>[4x]SYTLPSLPYAYDALEPHFDKQTMEIHHTKHHQTFVNNANAALESLPEFANLPVEELITKLDQLPADKKTVLRNNAGGHANHSLFWKGLKKG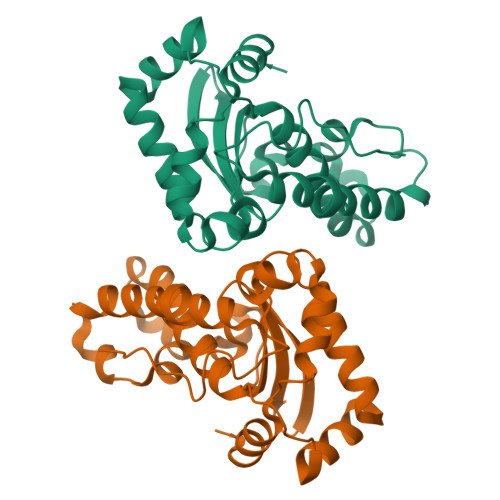TTLQGDLKAAIERDFGSVDNFKAEFEKAAASRFGSGWAWLVLKGDKLAVVSTANQDSPLMGEAISGASGFPIMGLDVWEHAYYLKFQNRRPDYIKEFWNVVNWDEAAARFAAKK>[2x]SSAAALPSPILNPDIPYNQLFINNEWQDAVSKKTFPTVNPTTGEVIGHVAEGDRADVDRAVKAAREAFRLGSPWRRMDASERGRLLNRLADLVERDRVYLASLETLDNGKPFQESYALDLDEVIKVYRYFAGWADKWHGKTIPMDGQHFCFTRHEPVGVCGQIIPWNFPLVMQGWKLAPALATGNTVVMKVAEQTPLSALYLASLIKEAGFPPGVVNIITGYGPTAGAAIAQHMDVDKVAFTGSTEV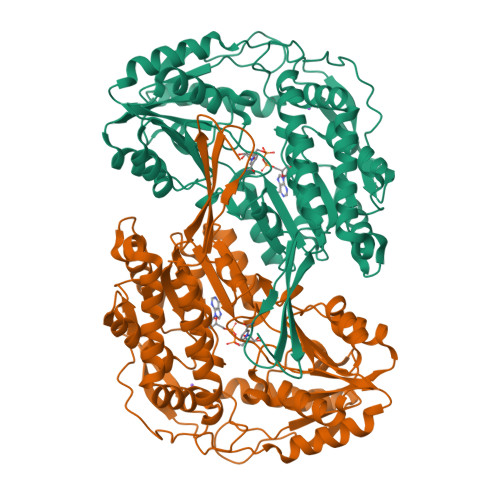GHLIQKAAGDSNLKRVTLELGGKSPSIVLADADMEHAVEQCHEALFFNMGQCCCAGSRTFVEESIYNEFLERTVEKAKQRKVGNPFELDTQQGPQVDKEQFERVLGYIQLGQKEGAKLLCGGERFGERGFFIKPTVFGGVQDDMRIAKEEIFGPVQPLFKFKKIEEVVERANNTRYGLAAAVFTRDLDKAMYFTQALQAGTVWVNTYNIVTCHTPFGGFKESGNGRELGEDGLKAYTEVKTVTIKVPQKNS> MKSSHHHHHHENLYFQSNAMENLGDKLSISQVYHLAQEYRDHAYSIANKIGSEEGLKQYYGLMNMSIQMFQLLKTKCTLSVLEDSKVTFEMVELLIQETYNFDLAELYISSLKERLQTHQSDTDLVEEIMRCEFLLLHDLPLMRDSKFHYKIALRNCNELVQYMVNLQDELYQNWASVFQYVGVMLCIKLKQHRRVKTSFHGLLSQCREKSQWKWFLNLCYVNYLLNERFPIPEDALQELRSTELHTVGPELYAWKLALEMVIQLCKDGNITDHLNEFKNFFDTNKQSLVTNEGKGCVIKIMPRIALKVELPMIFHYKELKNILLL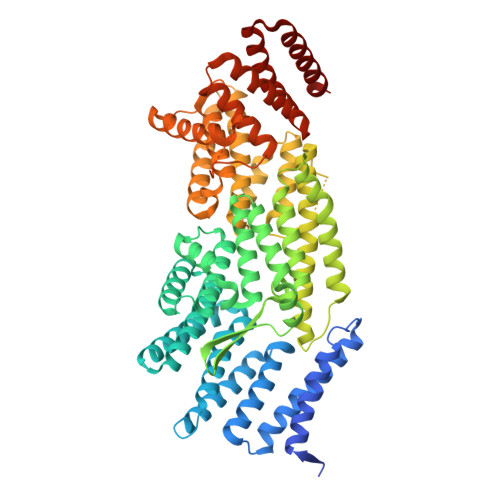LQSVSYIVNCYDEKGNFSRKFLPKVYSTTQKLIKNIAAGGVSMNELDSRIQTYKSILEFCEFYKVWEQTLLKGAVVTTESPKLGPSPGYVRLLQAMKVQFEGGGAVEEYTRLAQSGGTSSEVKMISLLNCYTVQAARVSRCSGDKQGELVEQCNKVWLQVEKLLQETDLQFNPIWECTVTILWLFSHFEPFSWNPLPCSDKQRAEYVSKLREFYSSNKFVAGEAVADNRFKLKKALLLQILVNYLGGRMLEHDLGEIYAISAKCFDMCRQQGGMRKVQYVIGIWHLMNCTVAMRGKDVALTNAKLEALVKQITSVKQ> GPLGSMVATVKRTIRIKTQQHILPEVPPVENFPVRQWSIEIVLLDDEGKEIPATIFDKVIYHLHPTFANPNRTFTDPPFRIEEQGWAGFPLDISVFLLEKAGERKIPHDLNFLQESYEVEHVIQIPLNKPLLTEELAKSGST

One of the major and widespread PTMs is acylation of the ε-amino group of lysine residues. Canonical acyllysine readers, bromodomain and double PHD finger (DPF), display comparable binding capabilities toward various short acyl chain modifications, and while the YEATS domain exhibits preference for crotonyllysine, it still associates albeit more weakly with other acyllysine marks. In this study, we elucidate the significance of π stacking components in targeting of acetyllysines by the YEATS domains and report a previously uncharacterized DNA-binding activity of the human AF9-YEATS domain. Collectively, our results have illuminated the mechanistic basis underlying distinct recognition of acyllysine PTMs by the YEATS domains of yeast Taf14 and human AF9, allowing us to develop a Taf14-YEATS module that selects for the crotonyl modification and discriminates against saturated acyl modifications.

To elucidate the mechanism by which Taf14-YEATS G82A distinguishes crotonyllysine and discriminates against saturated counterparts, we obtained the crystal structure of the H3K9cr-bound G82A mutant. The structure of the complex showed that the aromatic side chains of W81 and F62 lay parallel to each other and at equal distance of 3.4–3.6 Å from the crotonyl alkene group. Remarkably, only a single r2 conformation of W81 was observed in the structure of the complex. Analysis of molecular orbitals (MOs) for the W81, Kcr, and F62 assembly at the B3LYP/6-311 + G(d,p) level of density functional theory (DFT) revealed that the bonding MOs transcending all three π systems are deeply buried, indicating considerable synergism of the π-π-π stacking interaction. Given the taf14 G82A mutation impacts H3K9ac binding to a greater degree than H3K9cr binding, these findings suggest a differential requirement of H3K9ac and H3K9cr for the proper expression of Taf14-regulated genes.>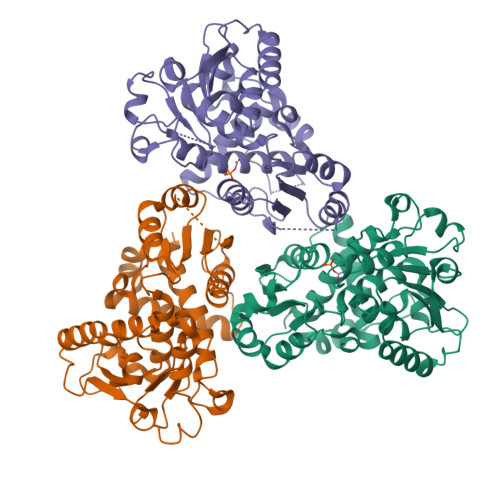[3x]MFYINSKYKIDLDKIMTKMKNKSVINIDDVDDEELLAILYTSKQFEKILKNNEDSKYLENKVFCSVFLEPSTATRCSFDAAILKLGSKVLNITDMNSTSFYAGETVEDAFKILSTYVDGIIYRDPSKKNVDIAVSSSSKPIINAGNGTGEHPTQSLLDFYTIHNYFPFILDRNINKKLNIAFVGDLKNGRTVHSLSKLLSRYNVSFNFVSCKSLNIPKDIVNTITYNLKKNNFYSDDSIKYFDNLEEGLEDVHIIYMTRIQKERFTDVDEYNQYKNAFILSNKTLENTRDDTKILHPLPRVNEIKVEVDSNPKSVYFTQAENGLYVRMALLYLIFSSTSAWSHPQFEK>[4x]MVKDEIVISSALRTPIGAFSGTLKDTPAAALGAHVVKTLLERTGLAPERVDEVVMGNVLQAGNGMNVARQVAVNGGLPVAVPAHTVNRVCGSGAQAVVTAYAQIRSGLSNLVIAGGVENMDQAPYLMPSLRHGARMGHTQALDALLRDGLNDAFSDQHSGWHTEDLVAKYEVSREAQDRFAATSQQRFAAAQAAGWFEGEIVPVTITTRKGETVFAKDEANRPD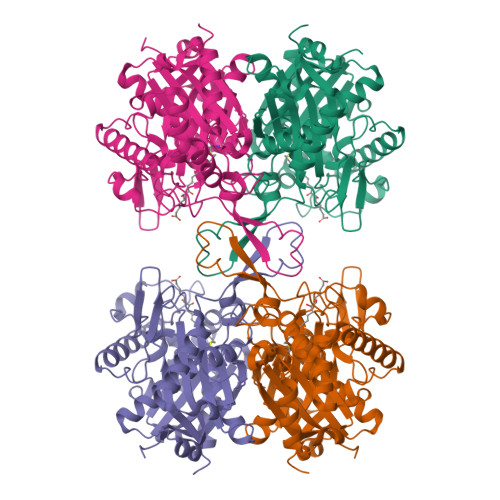TTEAGLAKLRPAFRKDGTITAGNAPGLNAGAAAMIVSSHATATELGLQPQLVIRGIGVAAVEPGLFGFGPVPAIKLALAQAQWQVQDVDRFEVNEAFAAVGLVVRDELGIAPERFNVDGGAIAHGHPIGATGAILLTKVAHALRRTSERRAVVSLCIGGGQGIALALERVKLAAALEHHHHHH> NISDTALTNELIHLLGHS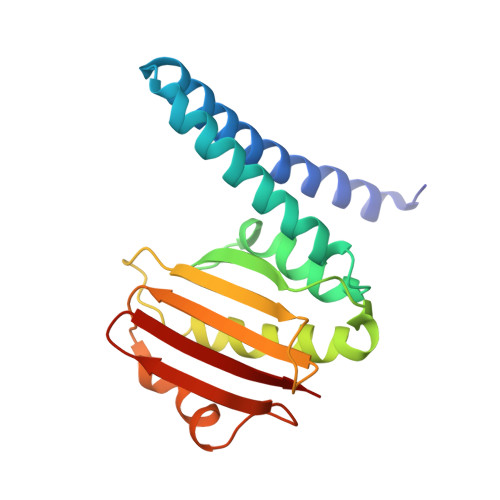RHDWMNKLQLIKGNLSLQKYDRVFEMIEEMVIDAKHESKLSNLKTPHLAFDFLTFNWKTHYMTLEYEVLGEIKDLSAYDQKLAKLMRKLFHLFDQAVSRESENHLTVSLQTDHPDRQLILYLDFHGAFADPSAFDDIRQNGYEDVDIMRFEITSHECLIEIGLD The cysteine desulfurase IscS is a highly conserved master enzyme initiating sulfur transfer via persulfide to a range of acceptor proteins involved in Fe-S cluster assembly, tRNA modifications, and sulfur-containing cofactor biosynthesis. IscS is a highly conserved, widely distributed pyridoxal-5′-phosphate (PLP)-dependent enzyme, with 60% sequence identity between the enzyme from Escherichia coli and its human homolog, NFS1. It initiates intracellular sulfur trafficking, delivering the sulfur to several sulfur-accepting proteins such as IscU, ThiI, TusA, and MoaD/MoeB that commit the sulfur to different metabolic pathways, including iron-sulfur cluster assembly, thiamine and biotin synthesis, tRNA modifications, or molybdopterin biosynthesis. The small domain (residues 1–15 and 264–404) contains the critical active site cysteine Cys328.

The IscS-TusA complex crystallized in two forms with identical heterotetramers consisting of an IscS dimer and two TusA molecules. TusA has a compact two-layered α/β-sandwich structure with a central four-stranded mixed β-sheet having the connectivity β1↑β2↑β4↓β3↑ and two α-helices. TusA interacts with the large domain of one IscS subunit within the dimer, with the exception of the tip of the loop containing the essential Cys328 of IscS, which comes from the other subunit. This persulfide-carrying Cys328IscS is juxtaposed against the acceptor cysteine of TusA, Cys19TusA, with only ∼4 Å separating their S atoms. Most of the IscS residues involved in the interaction with TusA are located on the outside face of a six-turn helix α2, the N-terminus of strand β2, the C-terminus of the neighbouring strand β9, and the following loop β9/α7. The residues of TusA contacting IscS are located on two α-helices (α1TusA and α2TusA), which are nearly perpendicular to helix α2IscS. Formation of the complex buries the α-helical layer of TusA and leaves its β-sheet layer exposed to the solvent. Approximately 710 Å2 of the molecular surface of each binding partner is buried, corresponding to ∼16% of the total TusA surface area. The main van der Waals contacts are provided by TusA Met24TusA, Met25TusA (α1TusA), Phe55TusA, Phe58TusA, Met59TusA (α2TusA) and IscS Trp45IscS (stacking with Phe58TusA), and the aliphatic portions of Arg55IscS and Arg237IscS. The conformation of the Cys328IscS loop in the IscS-TusA complex, with the donor and acceptor cysteines in close proximity, suggests that the observed conformation is close to that expected in a transfer-competent state.

>[2x]MGSSHHHHHHGSMYGVYRAMKLPIYLDYSATTPVDPRVAEKMMQFMTMDGTFGNPASRSHRFGWQAEEAVDIARNQIADLVGADPREIVFTSGATESDNLAIKGAANFYQKKGKHIITSKTEHKAVLDTCRQLEREGFEVTYLAPQRNGIIDLKELEAAMRDDTILVSIMHVNNEIGVVQDIAAIGEMCRARGIIYHVDATQSVGKLPIDLSQLKVDLMSFSGHKIYGPKGIGALYVRRKPRVRIEAQMHGGGHERGMRSGTLPVHQIVGMGEAYRIAKEEMATEMERLRGLRNRLWNGIKDIEEVYLNGDLEHGAPNILNVSFNYVEGESLIMALKDLAVSSGSACTSASLEPSYVLRALGLNDELAHSSIRFSLGRFTTEEEIDYTIELVRKSIGRLRDLSPLWEMYKQGVDLNSIEWAHH;>[2x]GSTDLFSSPDHTLDALGLRCPEPVMMVRKTVRNMQPGETLLIIADDPATTRDIPGFCTFMEHELVAKETDGLPYRYLIRKGG>SPKLKPWQKAFRQGRYAAAVDDVLNT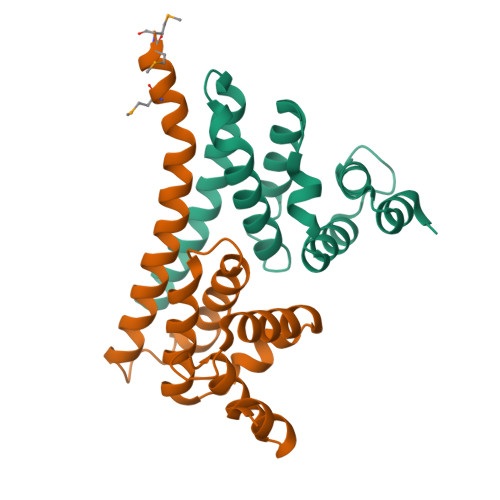TAPSYDPVIALTLLTALRHRSALREALQGRDELSVINILRWAGKYVADPRYRSICVDVAFHLIDLYAEHVGGSAELATQFQQLLAKVNREVEKAELAIVTGGMVESLMMSVEAQ[2x]>MQAKIKNKRVLVKFSGEALAGDNQFGIDIHVLDHIAKEIKSLVENDIEVGIVIGGGNIIRGVSAAQGGIIRRTSGDYMGMLATVINAVAMQEALEHIGLDTRVQSAIEIKEICESYIYRKAIRHLEKGRVVIFGAGTGNPF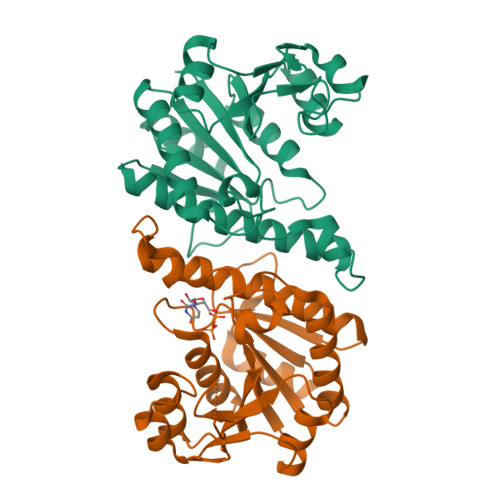FTTDTAATLRAIEIGSDLIIKATKVDGIYDKDPNKFKDAKKLDTLSYNDALIGDIEVMDDTAISLAKDNKLPIVVCNMFKKGNLLQVIKHQQGVFSMVK[6x]>[2x]MDPEFMSSVDVLLTVGKLDASLALLTTQDHHVIEFPTVLLPENVKAGSIIKMQVSQNLEEEKKQRNHFKSIQAKILEKYGTH;>MLSQTSIPEVKEDVIGYALHQRRARVGQFQDLGPPDLITLIKSLPSSSSTTTATASANDNGATSNINGQDPTTIVTELHSHDKLKGQIGTFFYCMGIDTSDPTSITIFAKKITDLFLDTPQIWFGKKKHFHVSKISISSWNAFRKYDVNIIVHIPGTVQTYIINSDGEQSQLPSVAEASSGRNSQDLNVNMIWAETFMSGIVRDIMIMKDNRADGESQNLVETLIFNPFTSGELEDVANNFIKLFPLVYEKGVYLDAPTHVLNPSLTNNYLVETLVEIVRLTKSLEACRKMLKKLIEIHPEAV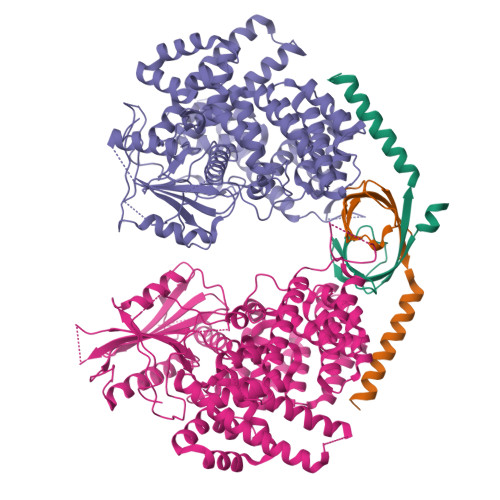IILIRVYFACDLEIDAVDLINEQLNSPSSFLADDSKTSHIQLIFKSELLSIQSEFLLDVKRDYKLAKEVAMEAVNCAPNEFKTWYLLTRIYIKLNDMSNALLSLNACPMSQVKEKYVLRRIAPITSDENLHLPLPLDASIEEISSLNPMDVQLEQKSADPNLVNLSASSLKSTFQLAYKLLTEIVQITGWEQLLKYRSKIFVMEDEYQGSTSSIDEAEVRGNDISKMRSKRLCERWLDNLFMLLYEDLKTYTDWQSEQLYFDAQNSKYHKLTVEWELFGLCAKRLGHLPEAAKAFQIGLSQRFSPVCAKNLLQFYIDEHKRIRRDSVSANSELTSSQILSSINDIDSSIIDLVVKICCWNHRWYIEFSIILIDALSVAVQDMGITKVHNEIASRFSDPVAQLIDDNILNFLKNFTNDTFDNGTENLYFQGHHHHHH[2x]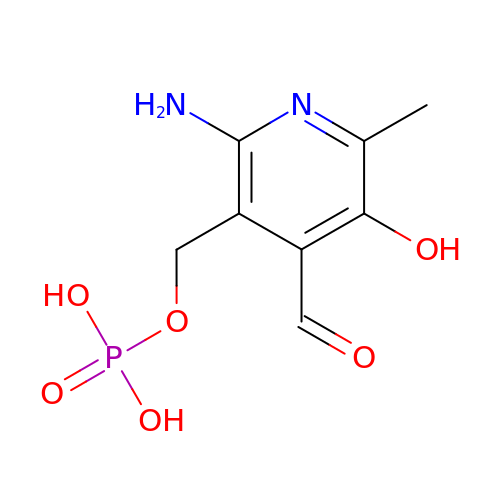(2-AMINO-4-FORMYL-5-HYDROXY-6-METHYLPYRIDIN-3-YL)METHYL DIHYDROGEN PHOSPHATE | C8 H11 N2 O6 P | XHTUTGLXZYJZRY-UHFFFAOYSA-N>[3x]MGSSHHHHHHSSGLVPRGSHQDPWKLSADKPDSNNYYGETVANGMIGIISSPEPLKVKEVVLAGTYDIYKRGRVSSFIPNYNLLNMKLAFNGESVQTYNINNYKQELDMRNGAFTGSFQFKDLATVTYSYYALRHLPHCIMMVVNINTQKDTEINVENLLETP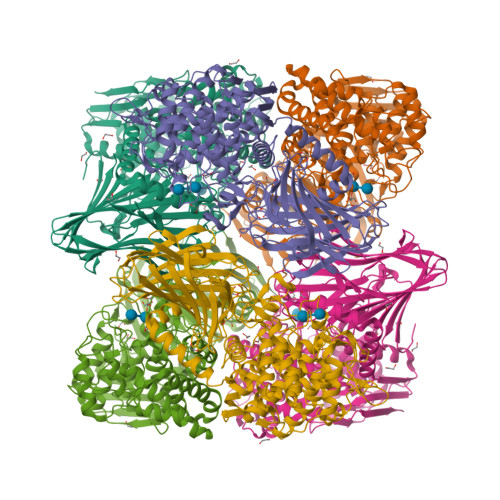SSLNNQQNYFQNITNTHVNIPLLTSVAFTPTGRSKIAVSNTFLFDEGKKLQPEILHRMNDADMHAMSFDKKIKAGKTYSFALIGSLISSDHINDPYNEAERLTIYAALEGKSRLLNRHMQEWNSLWQSDIQVEGDPQAQQDIRSMLYHLYSFTRKSTSLSPSPMGLSGLGYNGHVFWDTEIWMFPPMLLLHPEIAKSMIEYRYQRLDAARKKAAIYGYDGAMFPWESADSGAEETPVNALTGAFEHHVTGDVAIAAWQYYLVTGDKEWLKEKGWPILKATAEFWASRVEKNDKGEYEIKNVVAADEWAENIDNNAYTNGTAIRNLQYASKCATVLGVIAPKEWTLIADKILISKMSNGVTREHDSYTDQNIKQADANLLAYPLKLITDKEQIERDLKYYQTKIPQSDTPAMTQAIFSLLYSRLEDSDQAYHWFKDAYQPNLNPPFRVISECKGGTNPYFSTGAGGVLQAVIMGFGGLDIDAAGGIKQVKSVLPKNWKKLTITGIGIEKKTFVLTH> MVTVTDPLTARLEAAIKAWSDFFSDAEHERLDPAIFADQSQTLFANHPLAPVPLADLLLRPTPSNRECVDQRTLQYLQVLQKQGRITTAAVLRALYKYSTAHTRAQTPDGKPKHGAGDSS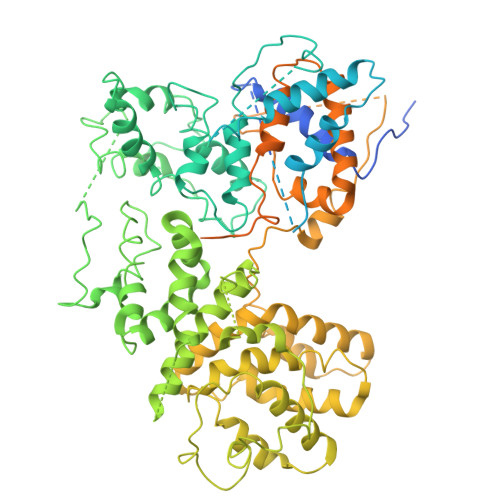TNDADVGGSSKADLTSRMVRWRNSYMVEEDVLWRLARAVNHGTGIKTSHDVTEVAKVLARWTALFAEVSAAISRDAFNSMNGLQVKDESEDARNAFVLFYFAFCENQIVNETLSQPVCKDICRKLLDSLDAFLPTLMHLTADITGRLEHFRSEVLARYAPQEKKSMDMPSFMNDLSMSLESFQVPELPVVNTRAGLYIYLGAALVGRPMIDDEALFSYLHNRYQGDLQAMAVHLILASFDLLANAVFRNEGAKTGHLLKSFLINKVPLILVQLVAYAATTMYPFNAEMCITEALNQVDINMFPTLSGMFDMPNNNSFNDSVRQDFCFACQLHGLLSQAAIETLLGDITYQSLPPEGRYVKEQLVQACLQEPDRTLKLIGELDNMNGNVGAAAQAIVEICRDLASKPLSLDVLLLFDKPHKILHPLCELLDNWAGYEEDHGEYQPVYEEFGSVLLLLLAFVYRYNLSTADLGIRSSGSFVAKLLNGVDRCQPLEQLSEQEKSHLGGWIHGLFDTEAGGLGDELMSSCPPQDFYLLAPTLFHQIVNALSAGYLTDEMLKGGLEYLVDVLLLPALVPALLYLSNLLWADNQPIQNAVIKILQPILKPTSISNEASTMLSSVLNIVAKPLEHALKSYQRQDPECQKIEPLLLAIADNLAVSRRTGGADHTELESWCSAQITNPATGALIHGGLAAAVRTTIQQLVQWAQNPTLNSMNGMPAPYTHRQTLAAQQILGPHRLLGIILDELKSSPEPGIAYDVVTTMICAPDVRNSTISSPSTQSNNSSDHNDQAQNHQSQDAKHKHPHRLTLRDALRLEAHDFRAHLRADPVLAETVVRLYRRVEAQLTPLALPLPPAAAAAPAVGVNVGVDAATAAAAAAAAAMMPDALGLGVVGGVELGGMEGAIAAAVAAANGSGTGGAGGDGTQGGAGDAGMGLDGQQQGQGGSSAGDMGLGGGTADDIFSGLSGPDDFGADFGSWSMDLS> AKCVSYGVAQIKAPALHSQGYTGSNVKVAVLDSGIDSSHPDLNVAGGASFVPSETNPFQDNNSHGTHVAGTVLAVAPSASLYAVKVLGADGSGQYSWIINGIEWAIANNMDVINMSL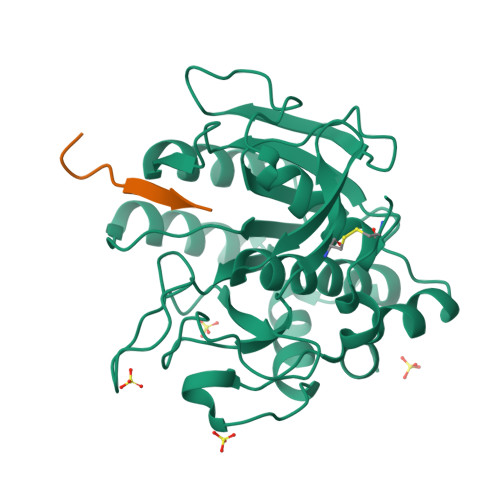GGPSGSAALKAAVDKAVASGVVVVAAAGNNGTSGSSSTVDYPAKYPSVIAVGAVDSSNQRAPWSSVGPELDVMAPGVSICSTLPGGKYGARSGTCGASNHVAGAAALILSKHPNWTNTQVRSSLENTATKLGDSFYYGKGLINVEAAAQHHHHHH;> VEEDHVAHA The studied chitin utilization locus (ChiUL) is encoded by the soil saprophyte Flavobacterium johnsoniae, which is a Bacteroidetes member exhibiting gliding motility. The ChiUL of F. johnsoniae consists of eleven genes that encode four enzymes, a predicted inner membrane transporter, a predicted two-component sensor/regulator system (TCS), and two individual SusC/D-like pairs (CusC/D, chitin utilization system). The SusC/D-like pairs are believed to be specific for their cognate carbohydrate targets, and act in concert to bind (SusD) and transport (SusC) oligosaccharides across the outer membrane. The resulting ChiOs, and likely chitin crystals as well (analogous to the archetypal starch-binding SusD protein of B. thetaiotaomicron), are captured by the CusD proteins.

CusDI and CusDII exhibit comparatively low sequence identity (27%) and may thus have different carbohydrate affinity characteristics. Isothermal calorimetry (ITC) studies with the recombinantly produced proteins revealed that CusDI binds the full range of tested oligomers (chitobiose to chitohexaose) with similar affinities, and even GlcNAc, though with much lower affinity. In this assay, CusDI displayed some enhanced affinity for chitotriose. Despite considerable efforts, crystals with bound ChiO ligands were not obtained, likely due to crystal packing, which for both proteins affected the predicted ligand-binding site. The overall structures of CusDI and CusDII overlay with an RMSD of 2.2 Å for 363 Cα pairs and display the canonical SusD protein fold featuring four tetratricopeptide repeats that act as a structural scaffold. The most striking feature of the putative substrate-binding regions of both CusDI and CusDII is the presence of two Trp residues that would provide a flat platform for binding ChiOs as well as insoluble chitin, as has been observed in chitin-binding carbohydrate-binding modules (CBMs). CusDI features W280 and W65, whereas CusDII displays W330 and W74 that are located at non-equivalent positions but may nevertheless have similar roles. While both glycan-binding platforms overlay within the known glycan-binding site of SGBP-A, they are offset from each other, suggesting that ChiOs are bound differently by each protein. The area of CusDI surrounding W280 and W65 displays several residues that may provide hydrogen-bonding or electrostatic interactions with individual GlcNAc residues of chitin, while there are fewer such residues within the aromatic interface of CusDII. This may account for the difference in binding specificity and affinity between the two proteins.

>MHHHHHHENLYFQGNGITLPDFEQDFNHIKGGFAPMFNNIQVLTPEWVYQLQQGLNSDIWSGYMATPTGFESGVNNTTYALLDNWNGFIWDYGYKNVMFNAYDIANKSKGKYDQFYALSLILKVEGMHRMTDTFGPIIYSKFGSNDATIAYDSQEEVYTQMFAELDTAVAELTKRIDAGEASTFESTDMTGYKGKYESWVRFANTLRLRLAMRIVKVKPALAKTEAEKAVAQKFGVMLVNDDSFKIVSPVYTNPIATISSSWLDIRMSADMESIMKGYQDPRIASYFDTSKQFPNEYKGVRTGIAISGKSDHQDFSGIGAVVRSKEIYLMNAAEAYFLRAEGALRGWNMGGTAQELYEAGIKASFDQRGVSGAAGYIADNTKTAAAYVDPNFPENNSDPVNNVTVAWDAAATNEVKLQKIITQKWIAGFPEGQEAWSDYRRTGYPKLFPVLKNYSGGAITTEFGVRRINFVQSEKAGNSGGVATGVSKLGGPDNGGTRVWWDVNAPNF[2x]P-NITRO-BENZYLAMINE | C7 H8 N2 O2 | 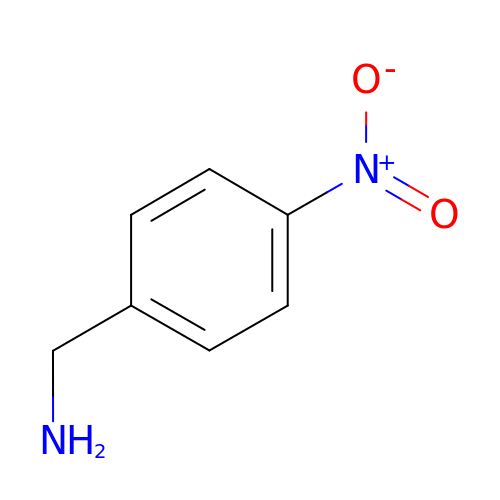ODVBBZFQPGORMJ-UHFFFAOYSA-N Rift Valley fever virus (RVFV; genus phlebovirus, family Phenuiviridae) is an important example of an enveloped virus that harbours a class II fusion protein. As with other phleboviruses, RVFV displays two glycoproteins on the lipid bilayer envelope of the virion, Gn and Gc, which form higher order pentameric and hexameric ring-shaped assemblies. While the Gc glycoprotein is responsible for membrane fusion, the role of the Gn remains undefined. Virus entry is completed upon Gc-mediated fusion of the viral envelope and host cell membrane, in a pH-dependent mechanism.

Localized reconstruction of each of the four types of the Gn–Gc capsomers (pentamers and hexamers of type 1–3) resulted in four independent structures at resolutions between 7.7 and 8.6-Å. Imposing lower than six-fold symmetry (two-fold symmetry for the type 2 hexamer and three-fold symmetry for the type 3 hexamer), or no symmetry (type 1 hexamer) gave the highest resolution, suggesting significant deviations from six-fold symmetry in the hexamers. We first performed fitting with the localized reconstruction of the pentamer at 7.7 Å resolution, followed by fitting the resulting Gn–Gc heterodimer model to localized reconstructions of the hexamers at 8.0–8.6 Å resolution. Consistent with previous biochemical and structural studies, this fitting verified that the Gn and Gc assemble as heterodimers, which form higher order ring-like pentameric and hexameric capsomer structures on the mature virion. Domain A of the Gn forms a ring on top of these capsomers interacting with domain II of Gc, occluding a surface area of ~950 Å2. The Gn–Gc interface is formed between the β-ribbon domain of the Gn and the hydrophobic fusion loops of Gc11, which are shielded from solvent at the interface between Gn domains A and B. As the N-linked glycosylation displayed on viruses is unlikely to be obscured in protein–protein interfaces, mapping of putative N-linked glycosylation sites onto pentameric and hexameric Gn–Gc capsomers was performed to validate the model. This analysis revealed all putative N-linked glycosylation sites to be either solvent exposed (RVFV Gn Asn438 and RVFV Gc Asn794, Asn1035) or facing unoccupied density that could partially correspond to an ordered glycan (Gc site Asn1077). Interestingly, the embedding of the fusion loops was only observed in the case of the pentamers and not with the hexamers.

>[6x]EDPHLRNRPGKGHNYIDGMTQEDATCKPVTYAGACSSFDVLLEKGKFPLFQSYAHHRTLLEAVHDTIIAKADPPSCDLQSAHGNPCMKEKLVMKTHCPNDYQSAHYLNNDGKMASVKCPPKYELTEDCNFCRQMTGASLKKGSYPLQDLFCQSSEDDGSKLKTKMKGVCEVGVQALKKCDGQLSTAHEVVPFAVFKNSKKVYLDKLDLKTEENLLPDSFVCFEHKGQYKGKLDSGQTKRELKSFDISQCPKIGGHGSKKCTGDAAFCSAYECTAQYANAYCSHANGSGIVQIQVSGVWKKPLCVGYERVVVKRELS;>DPGCSELIQASSRITTCSTEGVNTKCRLSGTALIRAGSVGAEACLMLKGVKEDQTKFLKIKTVSSELSCREGQSYWTGSFSPKCLSSRRCHLVGECHVNRCLSWRDNETSAEFSFVGESTTMRENKCFEQCGGWGCGCFNVNPSCLFVHTYLQSVRKEALRVFNCIDWVHKLTLEITDFDGSVSTIDLGASSSRFTNWGSVSLSLDAEGISGSNSFSFIESPGKGYAIVDEPFSEIPRQGFLGEIRCNSESSVLSAHESCLRAPNLISYKPMIDQLECTTNLIDPFVVFERGSLPQTRNDKTFAASKGNRGVQAFSKGSVQADLTLMFDNFEVDFVGAAVSCDAAFLNLTGCYSCNAGARVCLSITSTGTGSLSAHNKDGSLHIVLPSENGTKDQCQILHFTVPEVEEEFMYSCDGDERPLLVKGTLIAID[6x]3-[3-(3,3-DIMETHYLBUTANOYL)-1-(4-IODOBENZYL)-5-(QUINOLIN-2-YLMETHOXY)-1H-INDOL-2-YL]-2,2-DIMETHYLPROPANOIC ACID | C36 H37 I N2 O4 | 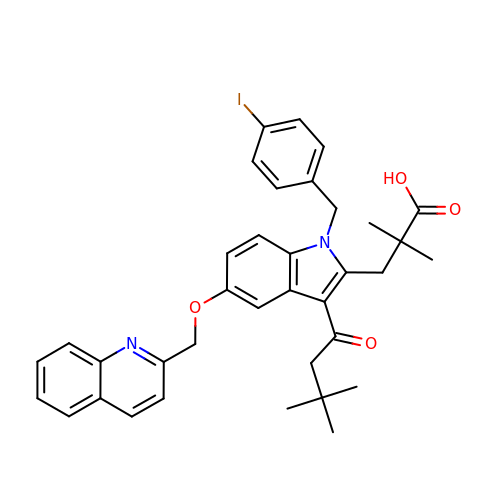VRDARPDCOSVXDY-UHFFFAOYSA-N>[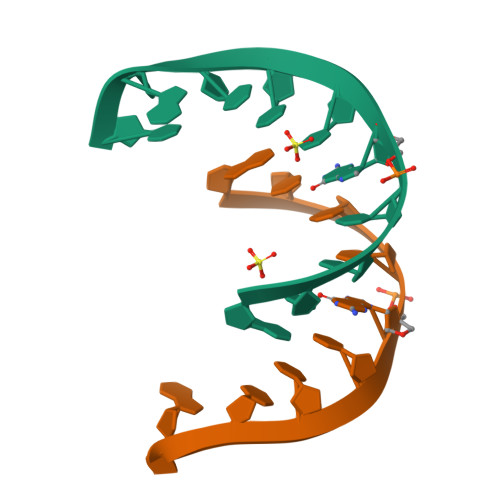2x]GCCUGCCUGC>KPIEIIGAPFSK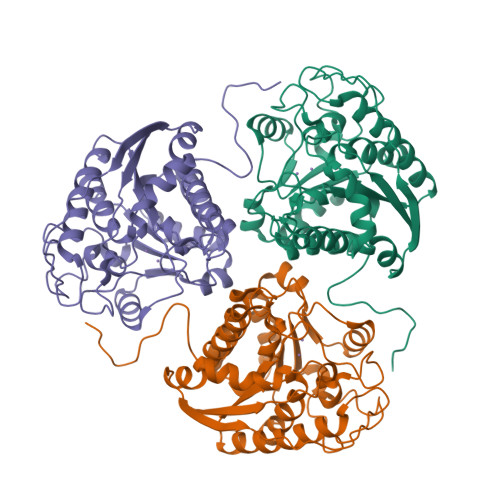GQPRGGVEKGPAALRKAGLVEKLKETEYNVRDHGDLAFVDVPNDSPFQIVKNPRSVGKANEQLAAVVAETQKNGTISVVLGGDHSMAIGSISGHARVHPDLCVIWVDAHTNINTPLTTSSGNLHGQPVAFLLKELKGKFPDVPGFSWVTPCISAKDIVYIGLRDVDPGEHYIIKTLGIKYFSMTEVDKLGIGKVMEETFSYLLGRKKRPIHLSFDVDGLDPVFTPATGTPVVGGLSYREGLYITEEIYKTGLLSGLDIMEVNPTLGKTPEEVTRTVNTAVALTLSCFGTKREGNHKPETDYL[3x]methyl (2S)-3-{4-amino-7-[(1E)-3-hydroxyprop-1-en-1-yl]-5-(4-methylphenyl)-7H-pyrrolo[2,3-d]pyrimidin-6-yl}-2-cyanopropanoate | C21 H21 N5 O3 | 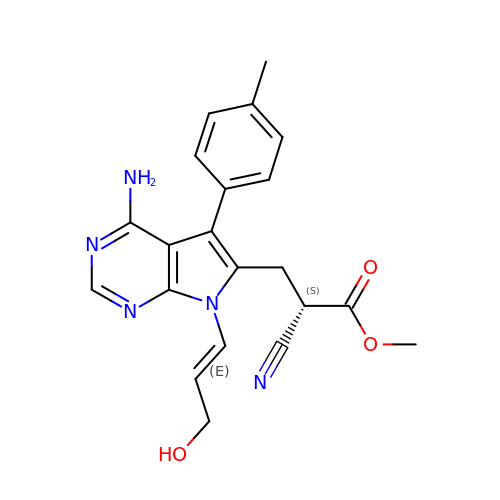ZJERBAYUHUAUBE-GZTQLTBSSA-N> MPKPINVRVTTMDAELEFAIQPNTTGKQLFDQVVKTVGLREVWFFGLQYVDSKGYSTWLKLNKKVTQQDVKKENPLQFKFRAKFFPEDVSEELIQEITQRLFFLQVKEAILNDEIYCPPETAVLLASYAVQAKYGDYNKEIHKPGYLANDRLLPQRVLEQHKLTKEQWEERIQNWHEEHRGMLR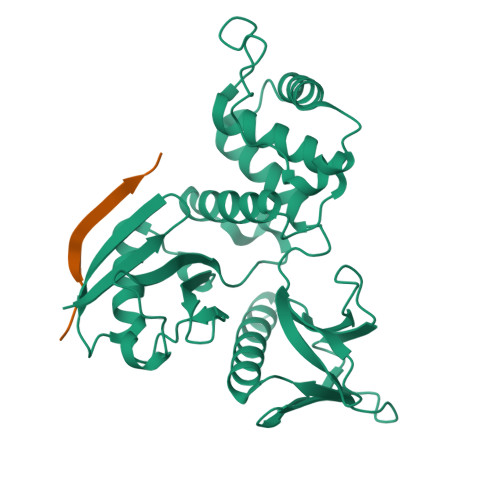EDSMMEYLKIAQDLEMYGVNYFEIKNKKGTELWLGVDALGLNIYEHDDKLTPKIGFPWSEIRNISFNDKKFVIKPIDKKAPDFVFYAPRLRINKRILALCMGNHELYMRRRK;> DSEPVLKGVKLHYT>[2x]MASGMIVTDAGADQPIVF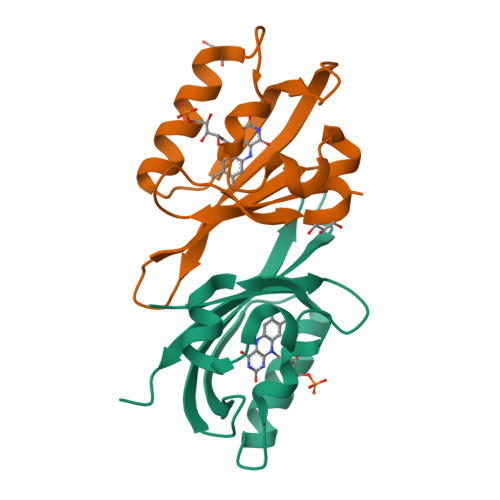VNRAFSTITGYAPNEVLGRNARFLQGPQTDAATVARLREAIAAARPIQERILNYRKDGQPFWNQLSISPVRDETGNVVAFVGVNTDVTAHHHHHH>ASAWPEEKNYHQPAILNSSALRQIAEGTSISEMWQNDLQPLLI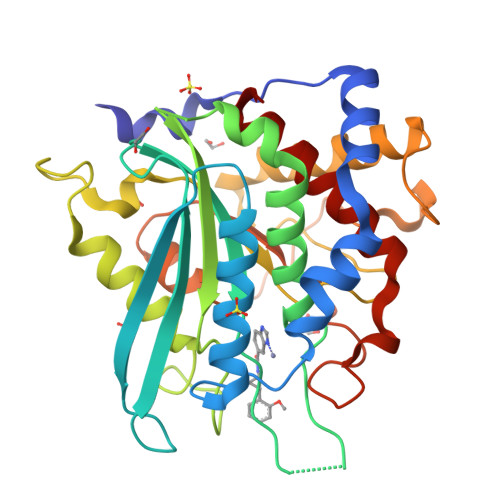ERYPGSPGSYAARQHIMQRIQRLQADWVLEIDTFLSQTPEGERSFSNIISTLNPTAKRHLVLACHYDSKYFSHWNNRVFVGATDSAVPCAMMLELARALDKKLLSLKTVSDSKPDLSLQLIFFDGEEAFLHWSPQDSLYGSRHLAAKMASTPHPPGARGTSQLHGMDLLVLLDLIGAPNPTFPNFFPNSARWFERLQAIEHELHELGLLKDHSLEGRYFQNYSYGGVIQDDHIPFLRRGVPVLHLIPSPFPEVWHTMDDNEENLDESTIDNLNKILQVFVLEYLHL[3x]> MEKYEELFARIKEKAKLIDEKIFELIPEKDPRVLYEAARHYPLAGGKRVRPFVVLTSTEAVGGDPLRAIYPAVAIELIHNYSLVHDDIMDMDETRRGKPTVHRIWGVNMAILAGDLLFSKAFEAVARAEIPPEKKARVLEVIVKASNELCEGQARDLEFEKKSTVTIEEYMEMISGKTGALFEASAKVGGIIGTDNEEYIKALSSWGRNVG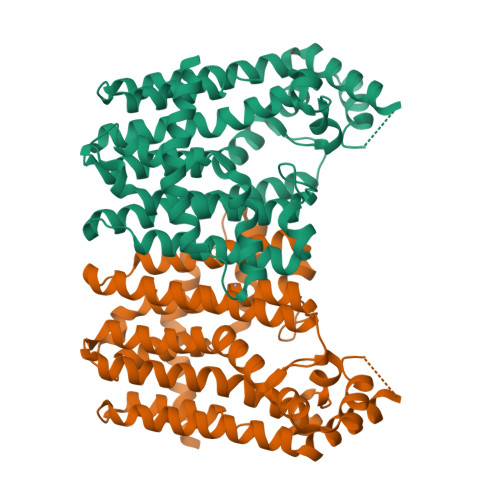IAFQIWDDVLDLIADEKKLGKPVGSDIRKGKKTLIVAHFFENADEKDKQRFLKIFGKYAGDVKGRGIIEEDIKSDVMEAIDLLKKYGSIDYAAEIAKDMIKKANEALRILPKSKARMDLELLAKFIVEREY>MRVLLIHSDYIEYEVKDKALKNPEPISEDMKRGRMEEVLVAFISVEKVDEKNPEEVSLKAIEEISKVAEQVKAENVFVYPFAHLSSELAKPSVAMDILNRVYQGLKERGFNVGKAPFGYYMAF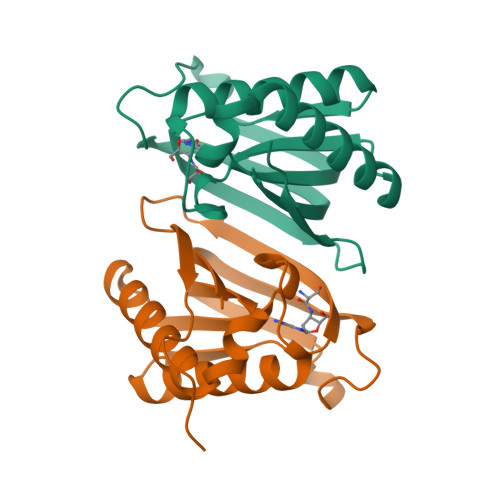KISCKGHPLAELSRTIVPEEARVE[2x]>DSISLSLINEGPSYASKVSVGSNKQQQTVIIDTGSSDFWVVDSNAQCGKGVDCKSSGTFTPSSSSSYKNLGAAFTIRYGDGSTSQGTWGKDTVTINGVSITGQQIADVTQTSVDQGILGIGYTSNEAVYDTSGRQTTPNYDNVPVTLKKQGKIRTNAYSLYLNSPSAETGTIIFGGVDNAKYSGKLVAEQVTSSQALTISLASVNLKGSSFSFGDGALLDSGTTLTYFPSDFAAQLADKAGARLVQVARDQYLYFIDCNTDTSGTTVFNFGNGAKITVPNTEYVYQNGDGTCLWGIQPSDDTILGDNFLRHAYLL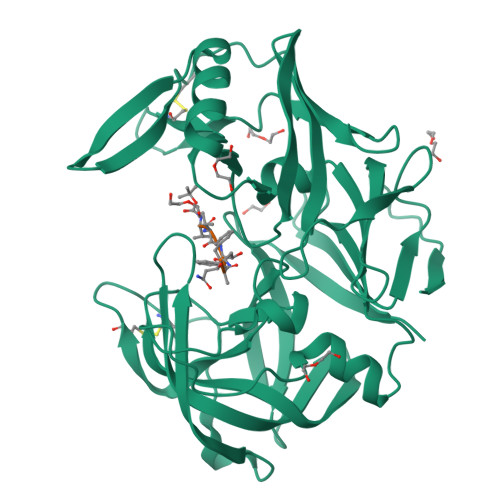YNLDANTISIAQVKYTTDSSISAV[4x];>XVVFAFA[4x]>EDVEIKPRGYQLRLVDHLTKSNGIVYLPTGSGKTFVAILVLKRFSQDFDKPIESGGKRALFMCNTVELARQQAMAVRRCTNFKVGFYVGEQGVDDWTRGMWSDEIKKNQVLVGTAQVFLDMVTQTYVALSSLSVVIIDECHHGTGHHPFREFMRLFTIANQTKLPRVVGLTGVLIKGNEITNVATKLKELEITYRGNIITVSDTKEMENVMLYATKPTEVMVSFPHQEQVLTVTRLISAEIEKFYVSLDLMNIGVQPIRRSKSLQCLRDPSKKSFVKQLFNDFLYQMKEYGIYAASIAIISLIVEFDIKRRQAETLSVKLMHRTALTLCEKIRHLLVQKLQDMTYDDDDDNVNTEEVIMNFSTPKVQRFLMSLKVSFADKDPKDICCLVFVERRYTCKCIYGLLLNYIQSTPELRNVLTPQFMVGRNNISPDFESVLERKWQKSAIQQFRDGNANLMICSSVLEEGIDVQACNHVFILDPVKTFNMYVQSKGRARTTEAKFVLFTADKEREKTIQQIYQYRKAHNDIAEYLKDRVLEKTEPELYEIKGHFQDDIDPFTNENGAVLLPNNALAILHRYCQTIPTDAFGFVIPWFHVLQEDERDRIFGVSAKGKHVISINMPVNCMLRDTIYSDPMDNVKTAKISAAFKACKVLYSLGELNERFVPKTLKERVASIADVHFEHWNKYGDSVTATVNKADKSKDRTYKTECPLEFYDALPRVGEICYAYEIFLEPQFESCEYTEHMYLNLQTPRNYAILLRNKLPRLAEMPLFSNQGKLHVRVANAPLEVIIQNSEQLELLHQFHGMVFRDILKIWHPFFVLDRRSKENSYLVVPLILGAGEQKCFDWELMTNFRRLPQSHGSNVQQREQQPAPRPEDFEGKIVTQWYANYDKPMLVTKVHRELTPLSYMEKNQQDKTYYEFTMSKYGNRIGDVVHKDKFMIEVRDLTEQLTFYVHNRGKFNAKSKAKMKVILIPELCFNFNFPGDLWLKLIFLPSILNRMYFLLHAEALRKRFNTYLNLHLLPFNGTDYMPRPLEIDYSLKRNVDPLGNVIPTEDIEEPKSLLEPMPTKSIEASVANLEITEFENPWQKYMEPVDLSRNLLSTYPVELDYYYHFSVGNVCEMNEMDFEDKEYWAKNQFHMPTGNIYGNRTPAKTNANVPALMPSKPTVRGKVKPLLILQKTVSKEHITPAEQGEFLAAITASSAADVFDMERLEILGNSFLKLSATLYLASKYSDWNEGTLTEVKSKLVSNRNLLFCLIDADIPKTLNTIQFTPRYTWLPPGISLPHNVLALWRENPEFAKIIGPHNLRDLALGDEESLVKGNCSDINYNRFVEGCRANGQSFYAGADFSSEVNFCVGLVTIPNKVIADTLEALLGVIVKNYGLQHAFKMLEYFKICRADIDKPLTQLLNLELGGKKMRANVNTTEIDGFLINHYYLEKNLGYTFKDRRYLLQALTHPSYPTNRITGSYQELEFIGNAILDFLISAYIFENNTKMNPGALTDLRSALVNNTTLACICVRHRLHFFILAENAKLSEIISKFVNFQESQGHRVTNYVRILLEEADVQPTPLDLDDELDMTELPHANKCISQEAEKGVPPKGEFNMSTNVDVPKALGDVLEALIAAVYLDCRDLQRTWEVIFNLFEPELQEFTRKVPINHIRQLVEHKHAKPVFSSPIVEGETVMVSCQFTCMEKTIKVYGFGSNKDQAKLSAAKHALQQLSKCDA[3x];> IDRYEQVSKDFEFIKI;>MEESMEELEALRRKKFTTYWELKEAGSVDHTGMRLCDRHNYFKNFYPTLKKEAIEAINSDEYESSKDKAMDVMSSLKITPKISEVESSSLVPLLSVELNCAFDVVLMAKETDIYDHIIDYFRTMLI[3x]

In Drosophila melanogaster, Dicer-2 (DmDcr-2)-mediated RNAi pathway plays important roles in defending against viral infections and protecting genome integrity. During the maturation of siRNAs, two cofactors can regulate DmDcr-2’s functions: Loqs-PD that is required for dsRNA processing, and R2D2 that is essential for the subsequent loading of siRNAs into effector Ago2 to form RISC complexes. Here we present several cryo-EM structures of DmDcr-2/R2D2/Loqs-PD complex bound to dsRNAs with various lengths by the Helicase domain. These structures revealed that R2D2 and Loqs-PD can bind to different regions of DmDcr-2 without interfering with each other.

In addition, from the 19-bp complex dataset, we obtained a trimer state structure with three DmDcr-2 molecules at a resolution of 3.70 Å. The structural comparison revealed that the arrangement of the DmDcr-2 molecules in the trimeric state is very similar to that of the dimeric state, but the RNA densities are discontinuous. This discontinuity resulted in variations in the bonding details between adjacent monomers. While dsRNA played a supportive role in the dimeric state, the DmDcr-2 monomers in the trimeric state exhibited much closer proximity to each other. This difference is further supported by the relative distances and angles between adjacent DmDcr-2 monomers, which were highly consistent in the trimeric state. In the 1st monomer of the quaternary complex of DmDcr-2/R2D2/Loqs-PD/19-bp siRNA, the presence of R2D2 does not affect the interaction of DmDcr-2 with Loqs-PD, as they bind to different sites. However, it is evident that only the 1st DmDcr-2 binds with Loqs-PD, while the same position in 2nd and 3rd DmDcr-2 is occupied by the “bridge helix” of R2D2. Therefore, although R2D2 and Loqs-PD do not overlap in binding position on a single DmDcr-2, R2D2 can occupy the binding position of Loqs-PD in the neighboring DmDcr-2 when the quaternary complexes form an oligomer. In the structure of the 19-bp complex, we also observe some density of the fourth DmDcr-2. Structural analysis indicates that the oligomeric mode of DmDcr-2 primarily depends on the dsRNA-induced conformational changes of the Helicase domain, independent of the length of dsRNA (19 bp or longer is sufficient). The trimeric structure of the complex allows for the full loading of siRNA duplexes into the Helicase domains, providing temporary protection against degradation until Ago2 is in close proximity.>[4x]MDAQYDISFADVEKAHINIRDSIHLTPVLTSSILNQLTGRNLFFKCELFQKTGSFKIRGALNAVRSLVPDALERKPKAVVTHSSGNHGQALTYAAKLE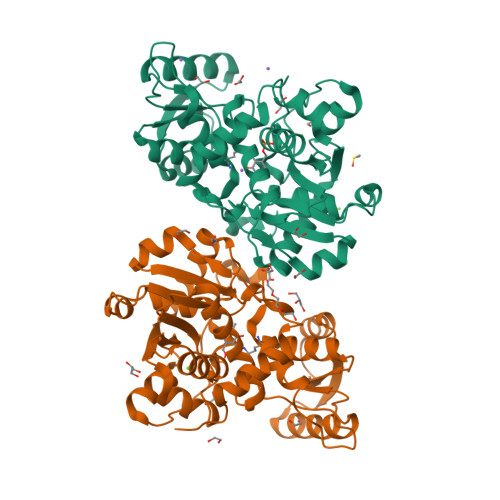GIPAYIVVPQTAPDCKKLAIQAYGASIVYCEPSDESRENVAKRVTEETEGIMVHPNQEPAVIAGQGTIALEVLNQVPLVDALVVPVGGGGMLAGIAITVKALKPSVKVYAAEPSNADDCYQSKLKGKLMPNLYPPETIADGVKSSIGLNTWPIIRDLVDDIFTVTEDEIKCATQLVWERMKLLIEPTAGVGVAAVLSQHFQTVSPEVKNICIVLSGGNVDLTSSITWVKQAERPASYQSVSVHHHHHH(3P)-3-(4-chloro-1H-imidazol-2-yl)-5-[(1R)-1-{[(3M)-3-(1H-pyrazol-5-yl)phenyl]oxy}ethyl]pyridine | C19 H16 Cl N5 O | 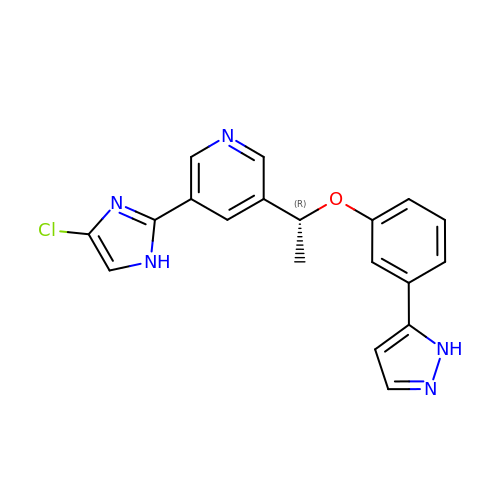FKQIJOHOBMULLA-GFCCVEGCSA-N The APOBEC3 family of enzymes (A3A-A3H) forms part of the innate immune response against viruses and transposons. The normally antiviral enzyme APOBEC3A is an endogenous mutagen in human cancer. Its single-stranded DNA C-to-U editing activity results in multiple mutagenic outcomes including signature single-base substitution mutations (isolated and clustered), DNA breakage, and larger-scale chromosomal aberrations. Here, we use X-ray crystallography to determine high-resolution structures of wildtype A3A/hairpin-inhibited complexes and demonstrate the underlying mechanism of inhibition.

Here we reveal the structural basis of competitive inhibition of wildtype APOBEC3A by hairpin DNA bearing 2′-deoxy-5-fluorozebularine in place of the cytidine in the TC substrate motif that is part of a 3-nucleotide loop. The hydroxyl group at C4 is coordinated to the Zn2+ center and is derived from the water/hydroxide ion bound to the Zn2+ in the substrate-free state. Tetrahedral coordination at the Zn2+ is completed by His70, Cys101, and Cys106. The catalytic glutamic acid residue, Glu72, which functions as a general acid/base, hydrogen bonds to C4-OH and N3-H of hydrated FdZ. The 5-fluoro group of FdZ is accommodated comfortably, abutting Tyr130. These results with wildtype A3A, together with prior work indicating hydration of dZ and its derivatives in structures with CDA and A3G, combine to demonstrate a universal mechanism of target nucleobase engagement, deamination, and inhibition.

>[2x]MEASPASGPRHLMDPHIFTSNFNNGIGRHKTYLCYEVERLDNGTSVKMDQHRGFLHNQAKNLLCGFYGRHAELRFLDLVPSLQLDPAQIYRVTWFISWSPCFSWGCAGEVRAFLQENTHVRLRIFAARIYDYDPLYKEALQMLRDAGAQVSIMTYDEFKHCWDTFVDHQGCPFQPWDGLDEHSQALSGRLRAILQNQGN>[4x]MDIISVALKRHSTKAFDASKKLTPEQAEQIKTLLQYSPSSTNSQPWHFIVASTEEGKARVAKSAAGNYVFNERKMLDASHVVVFCAKTAMDDVWLKLVVDQEDADGRFAT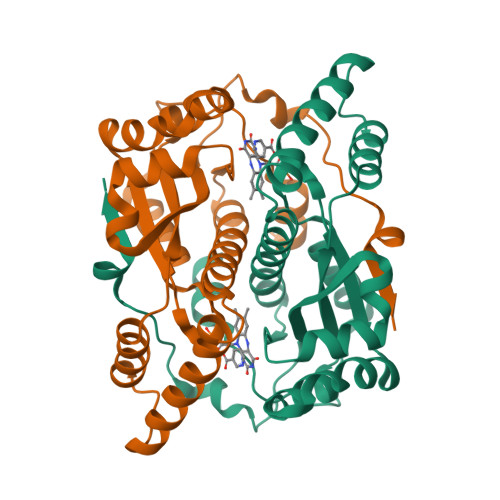PEAKAANDKGRKFFADMHRKDLHDDAEWMAKQVYLNVGNFLLGVAALGLDAVPIEGFDAAILDAEFGLKEKGYTSLVVVPVGHHSVEDFNATLPKSRLPQNITLTEV>ASRNQSSCDTVDQGYQCFSETSHLWGQYAPFFSLANESVISPEVPAGCRVTFAQVLSRHGARYPTDSKGKKYSALIEEIQQNATTFDGKYAFLKTYNYSLGADDLTPFGEQELVNSGIKFYQRYESLTRNIVPFIRSSGSSRVIASGKKFIEGFQSTKLKDPRAQPGQSSPKIDVVISEASSSNNTLDPGTCTVFEDSELADTVEANFTATFVPSIRQRLENDLSGVTLTDTEVTYLMDMCSFDTISTSTVDTKLSPFCDLFTHDEWINYDYLQSLKKYYGHGAGNPLGPTQGVGYANELIARLTHSPVHDDTSSNHTLDSSPATFPLNSTLYADFSHDNGIISILFALGLYNGTKPLSTTTVENITQTDGFSSAWTVPFASRLYVEMMQCQ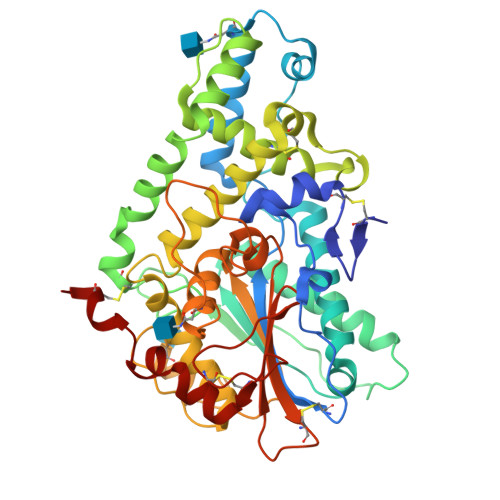AEQEPLVRVLVNDRVVPLHGCPVDALGRCTRDSFVRGLSFARSGGDWAECFA[2x]> APSTDPKSCPSVCRCDAGFIYCNDRSLTSIPVGIPEDATTLYLQNNQINNVGIPSDLKNLLKVQRIYLYHNSLDEFPTNLPKYVKELHLQENNIRTITYDSLSKIPYLEELHLDDNSVSAVSIEEGAFRDSNYLRLLFLSRNHLSTIPGGLPRTIEELRLDDNRISTISSPSLHGLTSLKRLVLDGNLLNNHGLG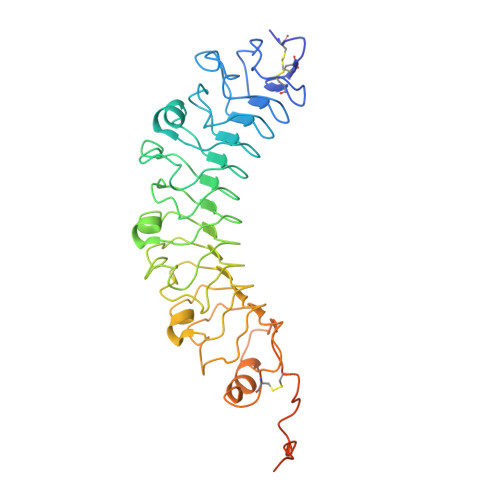DKVFFNLVNLTELSLVRNSLTAAPVNLPGTSLRKLYLQDNHINRVPPNAFSYLRQLYRLDMSNNNLSNLPQGIFDDLDNITQLILRNNPWYCGCKMKWVRDWLQSLPVKVNVRGLMCQAPEKVRGMAIKDLSAELFDCKDSGIVSTIQITTAIPNTAYPAQGQWPAPVTLEVLFQ>[2x]ATHTLQLAIGDEPTEGFDPMLGWSHGSYLLLHSPLLKQNEDFSWDSLLLSQYQPSDDGKTWLLTLKPDLKFSDGSPLTAKDVAFTYNNAAASGGKVDMGNFLSAEVIDPLNVRIHLKAPQSTFVNVLGSLGIVSADKYNAKTYAQKPIGAGPYRLVSFQPGQQMIVEANPYYAGNKNDFDKLIFVFLDEDSAFAAAQSGQLGVVRIPPSMAVGSVNNMKLWVRPSVENRGIVFPTTP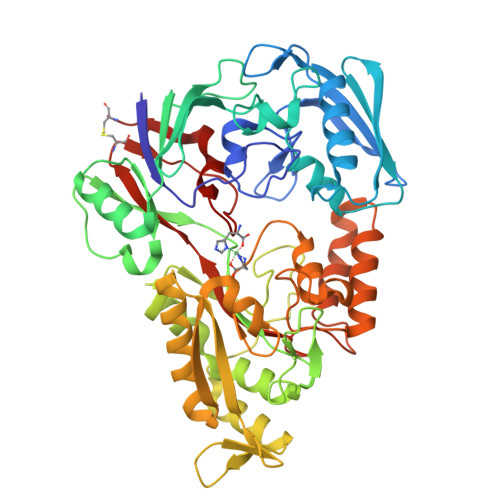AGKKDAHGYPIGNDVTADVAIRRAINYAINRQLLADQIMEGHAIPAYTGVQGLPWNNPDSAIKDGDIDKAKQILEQAGWQLNSQGTREKNGLPAKITLWYTSGDTTRRDLAQALRSMLKPIGIDVDLKSGSWETVERNMHANPTLFGWGSLDPMELYHHYSSNAAGVEYYNPGYYKNPMVDKHLQQALDAPTWQQAVPFWQQVDWDGTTGAGIRGDAAWAWLLNIQHTYLANNCVDLGKGTPEIHGSWSLLNSIDSWKWTCQ>MGSSHHHHHHSSGENLYFQGHMLEMTVNPITHYIGSFIDEFALSGITDAVVCPGSRSTPLAVLCAAHPDISVHVQIDERSAGFFALGLAKAKQRPVLLICTSGTAAANFYPAVVEAHYSRVPIIVLTADRPHELREVGAPQAINQHFLFGNFVKFFTDSALPEESPQMLRYIRTLASRAAGEAQKRPMGPVHVNVPLREPLMPDLS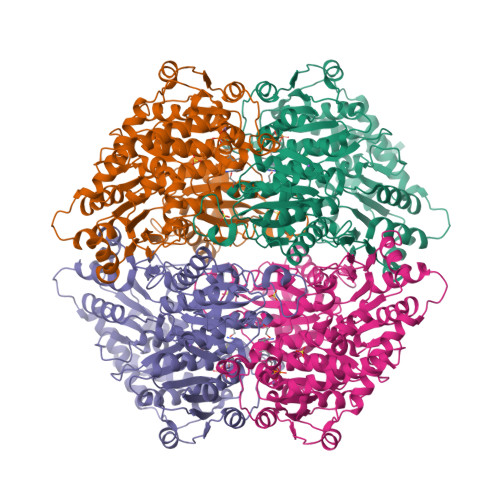DEPFGRMRTGRHVSVKTGTQSVDRESLSDVAEMLAEAEKGMIVCGELHSDADKENIIALSKALQYPILADPLSNLRNGVHDKSTVIDAYDSFLKDDELKRKLRPDVVIRFGPMPVSKPVFLWLKDDPTIQQIVIDEDGGWRDPTQASAHMIHCNASVFAEEIMAGLTAATRSSEWLEKWQFVNGRFREHLQTISSEDVSFEGNLYRILQHLVPENSSLFVGNSMPIRDVDTFFEKQDRPFRIYSNRGANGIDGVVSSAMGVCEGTKAPVTLVIGDLSFYHDLNGLLAAKKLGIPLTVILVNNDGGGIFSFLPQASEKTHFEDLFGTPTGLDFKHAAALYGGTYSCPASWDEFKTAYAPQADKPGLHLIEIKTDRQSRVQLHRDMLNEAVREVKKQWEL[4x]>[2x]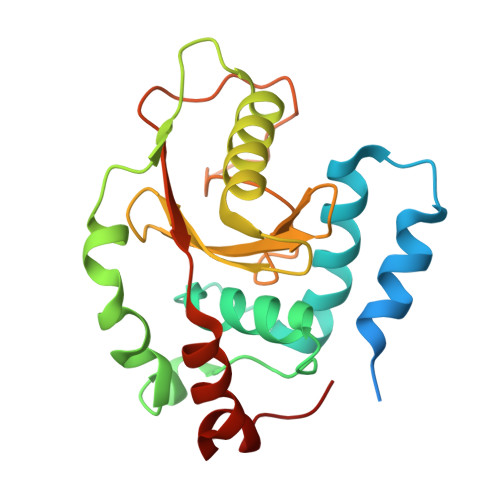GPLGSPEFMINGVSLQGTAGYEAHTEEGNVNVKKLLESLNSKSLGDMDKDSELAATLQKMINPSGGDGNASGCALHACMAMLGYGVREAPVPNEISEYMTGFFHRHLEQIDSEGIVSHPNETYSKFRERIAENILQNTSKGSVVMISIEQATHWIAGFNDGEKIMFLDVQTGKGFNLYDPVEKSPDAFVDENSSVQVIHVSDQEFDHYANSSSWKSKRLC>KKARMTVDKDYKIAEIDKRIYGSFVEHLGRAVYDGLYQPGNSKSDEDGFRKDVIELVKELNVPIIAYPGGNFVSNYFWEDGVGPVEDRPRRLDLAWKSIEPNQVGINEFAKWCKKVNAEIMMAVNLGTRGISDACNLLEYCNHPGGSKYSDMRIKHGVKEPHNIKVWCLGNAMDGPWQVGHKTMDEYGRIAEETARAMKMIDPSIELVACGSSSKDMPTFPQWEATVLDYAYDYVDYISLHQYYGNKENDTADFLAKSDDLDDFIRSVIATCDYIKAKKRSKKDIYLSFDEWNVWYHSNNEDANIMQNEPWRIAPPLLEDIYTFEDALLVGLMLITLMKHADRIKIACLAQLINVIAPIVTERNGGAAWRQTIFYPFMHASKYGRGIVLQPVINSPLHDTSKHEDVTDIESVAIYNEEKEEVTIFAVNRNIHEDIVLVSDVRGMKDYRLLEHIVLEHQDLKIRNSVNGEEVYPK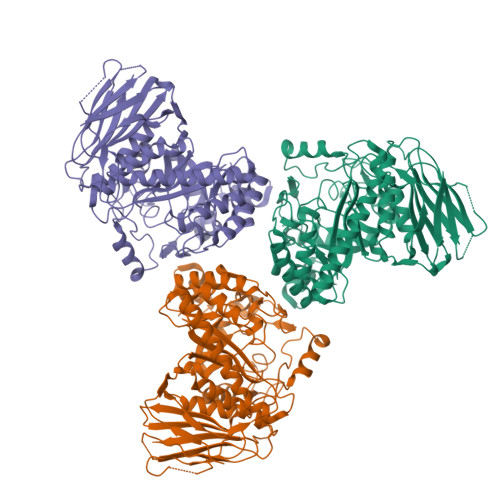NSDKSSFDDGILTSMLRRASWNVIRIG[6x]>GYTLWNDQIVKDEEVKIDKEDRGYQFGDGVYEVVKVYNGEMFTVNEHIDRLYASAEKIRITIPYTKDKFHQLLHELVEKNELNTGHIYFQVT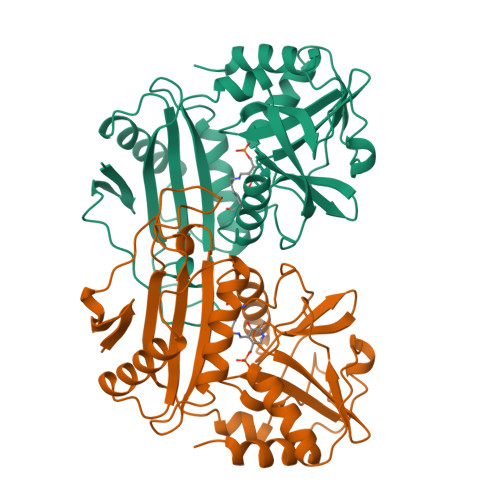RGTSPRAHQFPENTVKPVIIGYTKENPRPLENLEKGVKATFVEDIRWLRCDIKSLNLLGAVLAKQEAHEKGCYEAILHRNNTVTKGSSSNVFGIKDGILYTHPANNMILKGITRDVVIACANEINMPVKEIPFTTHEALKMDELFVTSTTSEITPVIEIDGKLIRDGKVGEWTRKLQKQFETKIP[2x]>MASNRKFFVGGNWKMNGSKESNQKLLKTLSDAKPDANTEILVAVPFVYLKDVREHLDKRFHVAAQNCYKVASGAFTGEISPAMIRDCGCEWVILGHSERRHIFGESDELIGEKVNHALTCGLKVVPCIGEKLDEREAGKTEQVCFRQLDAIKKGIPKAEDWSRVVIAYEPVWAIGTGKTASPEQAQEVHHAVRQWLEKNVSQAVASSLRITYGG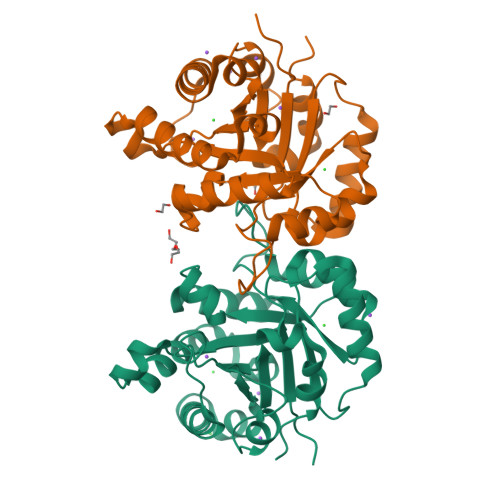SVTAANCKELAKKPDVDGFLVGGASLKPEFVDICNANRG[4x]>MDTSTTASVASANASTSTSMAYDLGSMSKDDVIDLFNKLGVFQAAILMFAYMYQAQSDLSIAKFADMNEASKESTTAQKMANLVDAKIADVQSSSDKNAKAQLPDEVISYINDPRNDITISGIDNINAQLGAGDLQTVKAAISAKANNLTTTVNNSQLEIQQMSNTLNLLTSARSDMQSLQYRTISGISLGK[50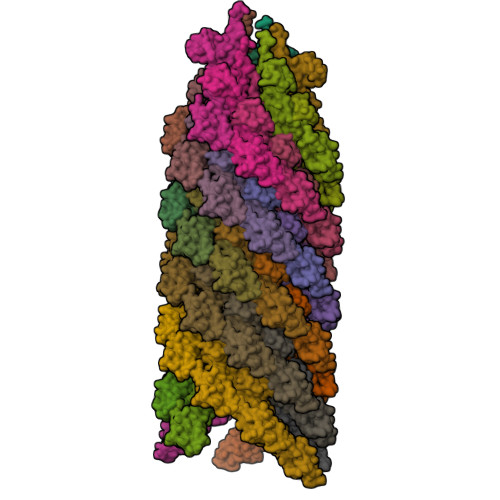x]>[2x]GPLGSEEDSAEAERLKTEGNEQMKVENFEAAVHFYGKAIELNPANAVY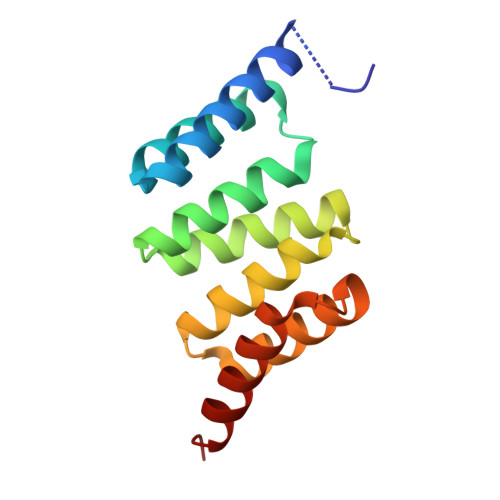FCNRAAAYSKLGNYAGAVQDCERAICIDPAYSKAYGRMGLALSSLNKHVEAVAYYKKALELDPDNETYKSNLKIAELKLREAP(4~{S})-5-[4-[[4-(2-ethyl-2-oxidanyl-butoxy)-2,3-dimethyl-phenyl]-dimethyl-silyl]-2,3-dimethyl-phenoxy]-4-oxidanyl-pentanoic 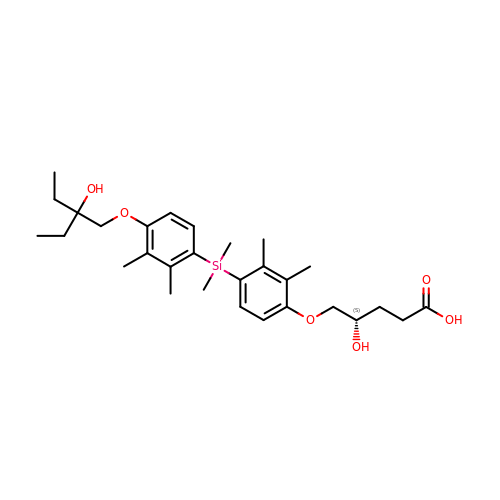acid | C29 H44 O6 Si | OUTAWAKGHUBDDX-HSZRJFAPSA-N> MSHITLDIAGQRSTLGIRRLRVQQLINEIPLAQLELHIPTDNHGAADNAVQHEVSRFTLGVRVGIAQDNKPLFDGYLVQKKMQLKGKEWSVRLEARHALQKLTFLPHSRVFRQQDDSTVMKGLLQSAGVKLTQESAAQLSSKHDQLLQFRLSDWQFIRSRLLSTNCWLLPDAASDTVVIRPLSDAAMASRTLARDSHDYTLYEINLNFDNRFTPDSLSLQGWDIAAQRLTAAQKSPAGAFRPWKPAGKVGQSSAGRQDYALAFSMLPEATLQTLSNSWLNYQQMTGVQGHIVLAGTRDFAPGESITLSGFGAGLDGTAMLSGVNQQFDTQYGWRSELVIGLPASMLEPAPPVRSLHIGTVAGFTADPQHLDRIAIHLPALNLPDSLIFARLSKPWASHASGFCFYPEPGDEVVVGFIDSDPRYPMILGALHNPKNTAPFPPDEKNNRKGLIVSQADQTQALMIDTEEKTLRLMAGDNTLTLTGEGNLTMSTPNALQLQADTLGLQADSN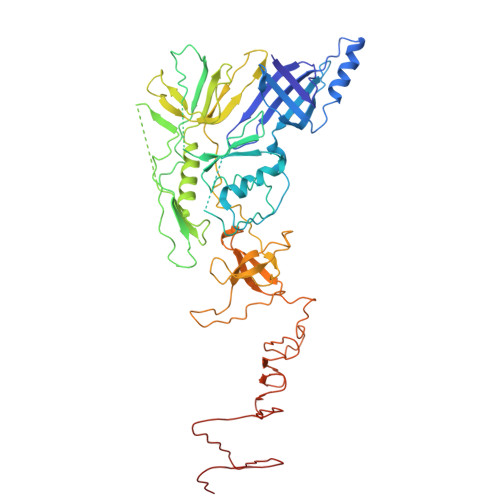LSIAGKQQVEITSAKINMKK> MAQNQRLTVVPTVTMLGVMKSRLVG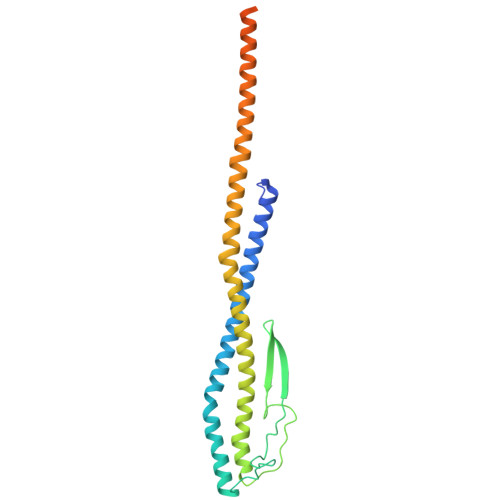ATRGHALLKKKSDALTVQFRQILKNIVTTKESMGEVMKDSSFALIEAKYVAGENIKHIVLENVQNASIKVRSRQENIAGVKIPKFEYFTDGETKNDLTGLARGGQQVQQCRAAYVKAIELLVELASLQTSFLTLDEAIKTTNRRVNALENVVKPRLENTITYIKGELDELEREDFFRLKKIQGYKKREIERQLASSKQFVEEQFAEKVSLQKGISIKSAQNLLSAGEKDEDIIF>MAHHHHHHSSGLEVLFQGPMTERLETRPQALLIKVPTEIVVKVVDDVDVAAPAVGQVGKFDDELYDEAGAQIGTSSGNFRIEYVRPTDGGLLTYYQ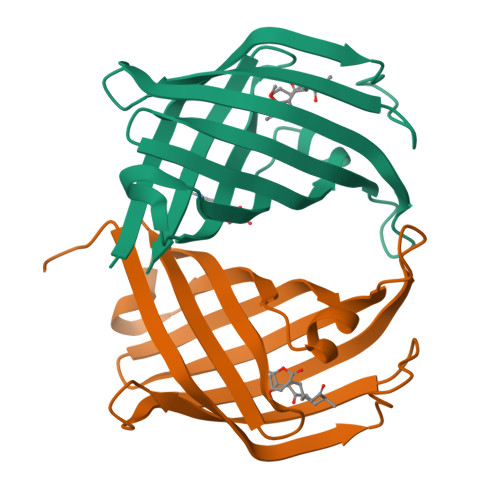EDITLSDGVIHAEGWADFNDVRTSKWVFYPATGVSGRYLGLTGFRQWRMTGVRKSAEARILLGE[4x]> GSHMSSLEKRLGKNEYFIITKSSPVRAILNDFAANYSIPVFISSSVNDDFSGEIKNEKPVKVLEKLSKLYHLTWYYDENILYIYKTNEISRSIITPTYLDIDSLLKYLSDTISVNKNSCN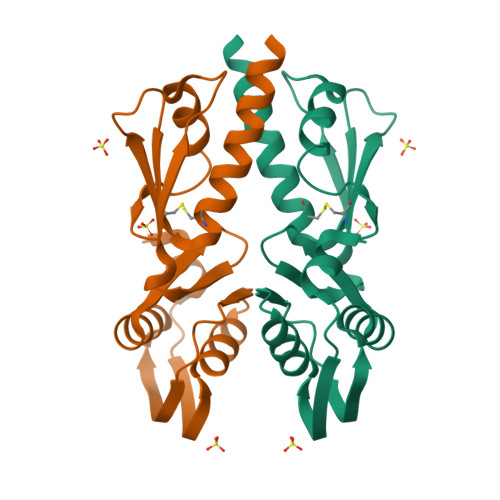VRKITTFNSIEVRGVPECIKYITSLSESLDKEAQSK> MSASSSSALPPLVPALYRWKSTGSSGRQVQRRCVGAEAIVGLEEKNRRALYDLYIATSLRNIAPASTLLTLQNLKEMFELALLDARFEHPECACTVSWDDEVPAIITYESPES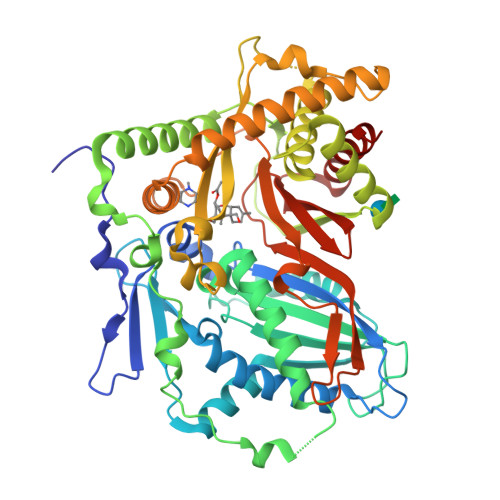NESARDWARGCIHVQPTAKSALDLWSEMEEGRAAANDNTPSKSIELFLLSDVSTDSTPIPQDATVEILFHSNHLFWDGIGCRKFVGDLFRLVGSYIGRSDSREMKKIQWGQEIKNLSPPVVDSLKLDINTLGSEFDDKCTEYTSALVANYKSRGMKFQPGLALPRCVIHKLSADESIDIVKAVKTRLGPGFTISHLTQAAIVLALLDHLKPNDLSDDEVFISPTSVDGRRWLREDIASNFYAMCQTAAVVRIENLKSITVSHKDEKELQVRALESACRNIKKSYRQWLENPFLQALGLRVHNFEASYLHAKPIPFEGEANPLFISDGINERFIPHEIKQTATGENVLSVESIDFVVNQSLPYLAIRLDSWRDASTLNIIYNDANYTEAEVQKYLQSIVEFMLAFRL Here, we study fold transition between distinct β-barrels by protein engineering and structural biology technique. Here, we discover that the previously reconstructed ancient DPBB sequence could also adopt a β-barrel fold named Double-Zeta β-barrel (DZBB), as a metamorphic protein. The DZBB fold is not found in any modern protein, although its structure shares similarities with RIFT and OB. Furthermore, the reconstructed OB fold could also be converted to the four-stranded SH3 fold by a simple circular permutation. Thus, these ancient β-barrel folds (DPBB, RIFT, OB, and SH3) could be readily interconverted by a few feasible mutations through the missing-link fold, DZBB, indicating their significantly close evolutionary relationships.

E The remodeling of the loop connecting β1-β2 in design-2 resulted in the RIFT-fold protein, design-3. CD experiments demonstrated that design-3 and design-5 were partially folded, and design-3 formed well-diffracting crystals. The crystallographic analysis revealed that design-3 and design-4 adopted the homo-dimeric RIFT-fold. Thus, the short In/Del at the 1st loop position is the determinant for the fold transition between DZBB and RIFT. A single deletion in the DZBB sequence converted it into the RIFT fold. Most DNA molecules did not migrate from the well when mixed with the proteins with the stable DZBB fold (design-2, -18, and -19) and RIFT fold (design-3 and -4), indicating that these proteins formed large aggregates with dsDNA. Design-2 seems to have a higher affinity for dsDNA than design-3, as dsDNA shifted even at lower concentrations of design-2.

> GPMPGKKFVARVAEADGKRVVIIPKAERAKVGIKVGDVVEVKKV> GSARNHTEDNSTEYYDYEEARCACPARHLNNTNGTVLKLLGCHYFCNGTLCTAPDGYPCYNLTAQQVRTLTTYPNTSCAVGVCMKGTCVKNGTMEQCFKTP;> ARGTNVGRECCLEYFKGAIPLRKLKTWYQTSEDCSRDAIVFVTVQGRAICSDPNNKRVKNAVKYLQSLERS

Evasins are chemokine-binding proteins from tick saliva, whose application as anti-inflammatory therapeutics will require manipulation of their chemokine target selectivity. Here we describe subclass A3 evasins, which are unique to the tick genus Amblyomma and distinguished from “classical” class A1 evasins by an additional disulfide bond near the chemokine recognition interface. The A3 evasin EVA-AAM1001 (EVA-A) bound to CC chemokines and inhibited their receptor activation. Structures of chemokine-bound EVA-A revealed a deep hydrophobic pocket, unique to A3 evasins, that interacts with the residue immediately following the CC motif of the chemokine.

To understand how class A3 evasins achieve chemokine binding and inhibition, we purified and crystallised complexes of EVA-A bound to human CCL7, CCL11, CCL16 and CCL17, and solved their structures at resolutions of 1.51–2.01 Å. All four structures display the same fold and 1:1 stoichiometry. EVA-A displays a rigid core structure comprised of seven β-strands and one α-helix, stabilised and interconnected by five disulfide bonds. In the EVA-A:chemokine structures, the side chain of the chemokine CC + 1 residue (Tyr in CCL7; Phe in CCL11, Leu in CCL16 and CCL17) sits in a deep hydrophobic pocket within the evasin structure, possibly enabling the ~35° rotation of the chemokine relative to its position in class A1 evasin complexes. Previously, structures have been reported for the class A1 evasin EVA-P974 (hereafter abbreviated to EVA-P) bound to CCL7 and CCL17. Comparison of these to our structures of EVA-A bound to the same chemokines enabled us to identify similarities and distinctive aspects of chemokine recognition by class A3 evasins. On the other hand, there is a consistent ~35° rotation of the chemokine between the available class A1 and class A3 evasin-bound structures, suggesting that class A3 evasins enable closer interactions with the N-loop region of the chemokine. Moreover, the inter-chain positions between CCL17 and EVA-A exhibited less variability than that between CCL17 and EVA-P, suggesting a more stable complex formed between CCL17 and EVA-A. This is consistent with EVA-A forming high-occupancy hydrogen bonds with CCL17 residues Cys50 and Asp33, thus “clamping” each end of the CC motif region. However, upon binding to CCL17, EVA-A became more rigid (lower root-mean-square fluctuation (RMSF) values) than EVA-P. The observation that EVA-A is more flexible in the free state but more rigid in the chemokine-bound state, in comparison to EVA-P, is consistent with EVA-A forming tighter interactions. This is further supported by the lower flexibility of CCL17 and the increased frequency of high-occupancy hydrogen bonds for the class A3 evasin:chemokine complex.>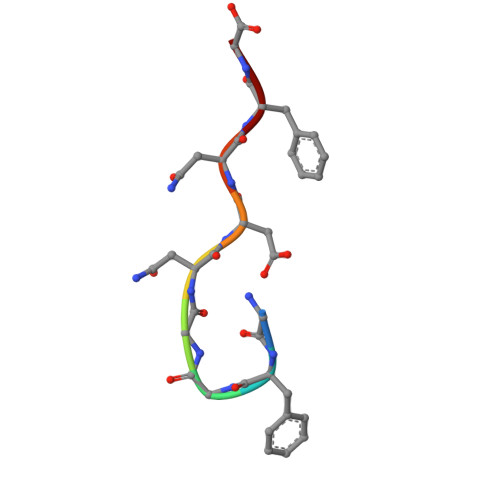 GFGGNDNFG(2~{Z},4~{E})-3-cyclopropyl-5-[(1~{S})-2,6,6-trimethyl-1-oxidanyl-4-oxidanylidene-cyclohex-2-en-1-yl]penta-2,4-dienoic 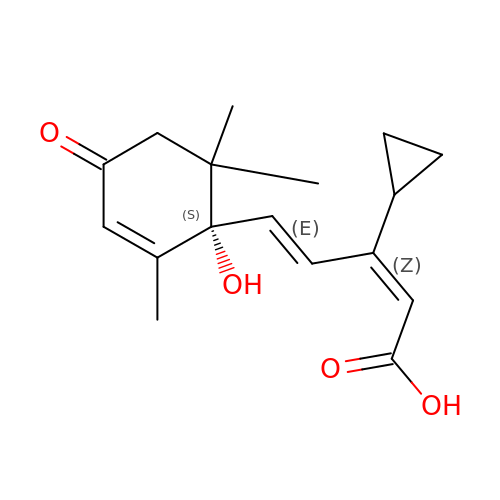acid | C17 H22 O4 | HKEUSUYMMUPOQP-PZUGTFMISA-N> MGDHANEQIIDMPENSEMKSMKNDAFSQAKFAVENYKFENKISSHIKKFFDEKYGPNWHCVVGKHFNAYVSYDSKN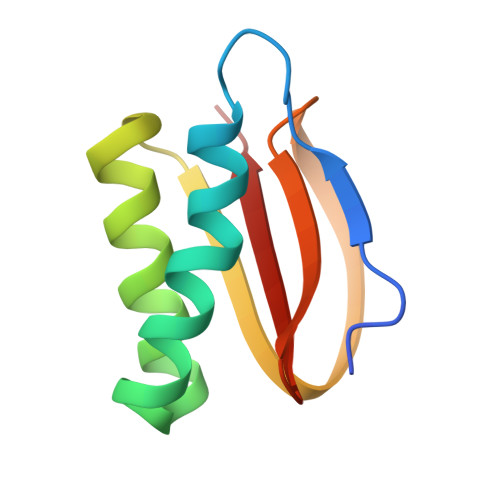FIFFYEGQLAILLYRKG> SASEEQVAQDTEE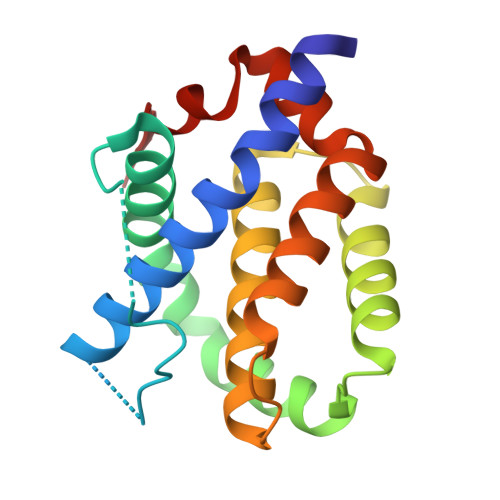VFRSYVFYRHQQEQEAEGVAAPADPEMVTLPLQPSSTMGQVGRQLAIIGDDINRRYDSEFQTMLQHLQPTAENAYEYFTKIATSLFESGINWGRVVALLGFGYRLALHVYQHGLTGFLGQVTRFVVDFMLHHSIARWIAQRGGWVAALNLCNG>[4x]MADGEKRVQVAGVIGTN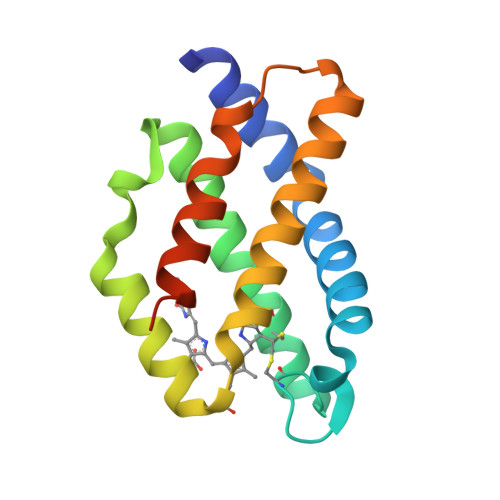AAEVVKTAVSQLFQEYPELVRPGGCAYTTRRYNMCVRDMNYFLRMCSYAIVAGGASVLDERMLAGFRDTFNSLGIPLCPTARSIQLMKKIVKEKLATAGMTNIAFVDEPFDYIARVISETEILEHHHHHH6-ethyl-5-{(3S)-3-[3-(isoquinolin-5-yl)-5-methoxyphenyl]but-1-yn-1-yl}pyrimidine-2,4-diamine 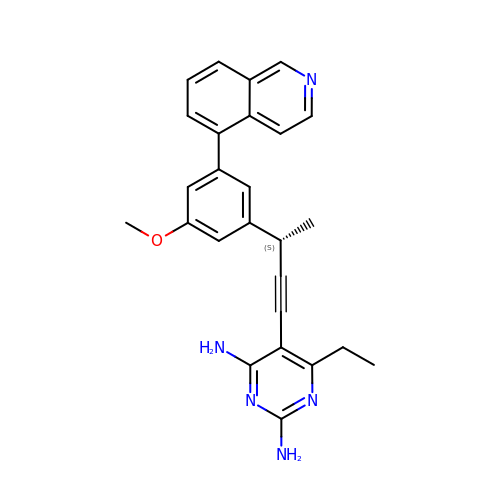| C26 H25 N5 O | MGLLCDAARSVGLO-MRXNPFEDSA-N>[4x]RVVCREASHAGSWYTASGPQLNAQLEGWLSQVQSTKRPARAIIAPHAGYTYCGSCAAHAYKQVDPS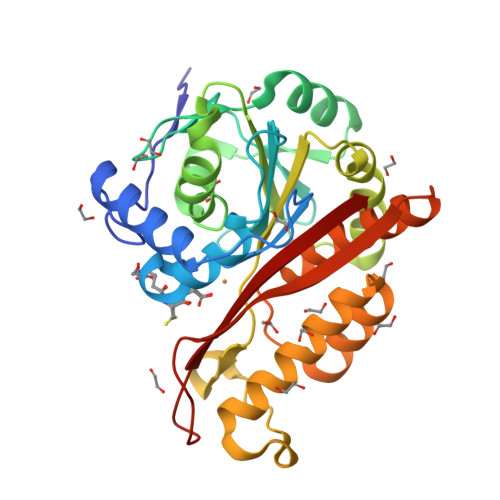ITRRIFILGPSHHVPLSRCALSSVDIYRTPLYDLRIDQKIYGELWKTGMFERMSLQTDEDEHSIEMHLPYTAKAMESHKDEFTIIPVLVGALSESKEQEFGKLFSKYLADPSNLFVVSSDFCHWGQRFRYSYYDESQGEIYRSIEHLDKMGMSIIEQLDPVSFSNYLKKYHNTICGRHPIGVLLNAITELQKNGMNMSFSFLNYAQSSQCRNWQDSSVSYAAGALTVH>ETPVLEKNNVTLTGGGENVTKELKDKFTSGDFTVVIKYNQSSEKGLQALFGISNSKPGQQNSYVDVFLRDNGELGMEA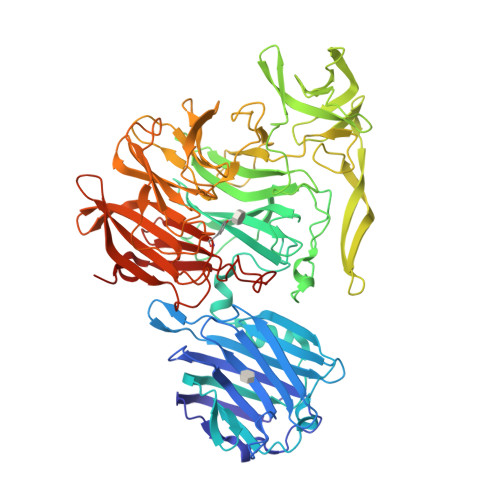RDTSSNKNNLVSRPASVWGKYKQEAVTNTVAVVADSVKKTYSLYANGTKVVEKKVDNFLNIKDIKGIDYYMLGGVKRAGKTAFGFNGTLENIKFFNSALDEETVKKMTTNAVTGHLIYTANDTTGSNYFRIPVLYTFSNGRVFSSIDARYGGTHDFLNKINIATSYSDDNGKTWTKPKLTLAFDDFAPVPLEWPREVGGRDLQISGGATYIDSVIVEKKNKQVLMFADVMPAGVSFREATRKDSGYKQIDGNYYLKLRKQGDTDYNYTIRENGTVYDDRTNRPTEFSVDKNFGIKQNGNYLTVEQYSVSFENNKKTEYRNGTKVHMNIFYKDALFKVVPTNYIAYISSNDHGESWSAPTLLPPIMGLNRNAPYLGPGRGIIESSTGRILIPSYTGKESAFIYSDDNGASWKVKVVPLPSSWSAEAQFVELSPGVIQAYMRTNNGKIAYLTSKDAGTTWSAPEYLKFVSNPSYGTQLSIINYSQLIDGKKAVILSTPNSTNGRKHGQIWIGLINDDNTIDWRYHHDVDYSNYGYSYSTLTELPNHEIGLMFEKFDSWSRNELHMKNVVPYITFKIEDLKKNL[2x]> MGSD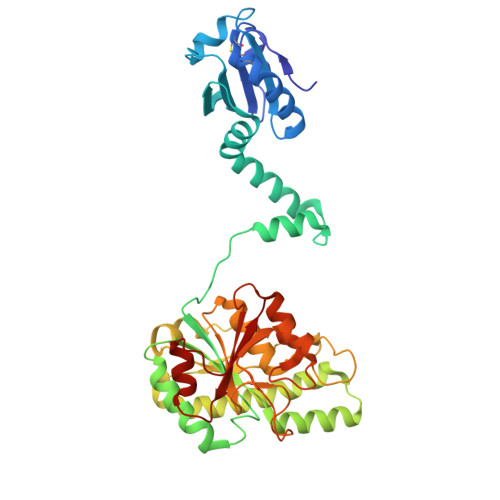KIIHLTDDSFDTDVLKADGAILVDFWAEWCGPCKMIAPILDEIADEYQGKLTVAKLNIDQNPGTAPKYGIRGIPTLLLFKNGEVAATKVGALSKGQLKEFLDANLEEEKRKREEELLMQRSLTDPQLQAAAAAAADFRILPDATVIKIGGQSVIDRGRAAVYPLVDEIVAARKNHKLLIGTGAGTRARHLYSIAAGLGLPAGVLAQLGSSVADQNAAMLGQLLAKHGIPVVGGAGLSAVPLSLAEVNAVVFSGMPPYKLWMRPAAEGVIPPYRTDAGCFLLAEQFGCKQMIFVKDEDGLYTANPKTSKDATFIPRISVDEMKAKGLHDSILEFPVLDLLQSAQHVREVQVVNGLVPGNLTRALAGEHVGTIITAS> DFVERQQWLAQPPQKEIPDLELPVGLVIALPTNSENCSTQAICVLRVRLLQTYDIESSQKCDIAYNFLIGGDGNVYVGRGWNKMGAHMNNINYDSQSLSFAYIGSFKTIQPSAKQLSVTRLLLERGVKLGKIAPSYRFTASSKLMPSVTDFKADALYASFANWTHWS;> MVILKVAEWGGRPAKRMLDAQQLPINRVVISHTAAEGCESREVCSARVNVVQSFHMDSWGWDHIGYNFLVGGDGRVYEGRGWDYVGAHTKGYNRGSIGISFIGTFTTRKPNERQLEACQLLLQEGVRLKKL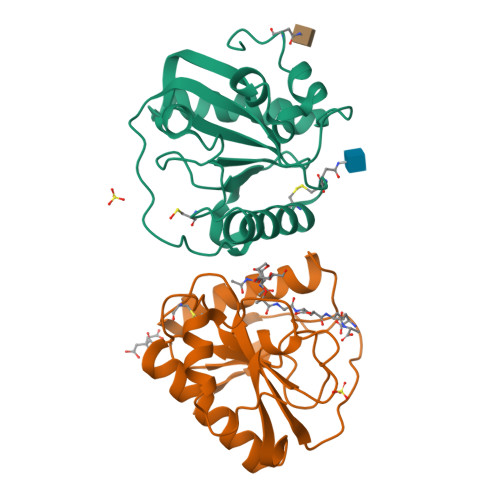TTNYRLYGHRQLSATESPGEELYKIIKKWPHWSHEI During infection the influenza A virus NS1 protein participates in multiple protein-RNA and protein-protein interactions to perform a plethora of functions. The N-terminal 73 amino-acid residues of NS1 form a symmetrical homodimeric RNA-binding domain (RBD), which is connected to the central effector domain (ED; residues 86-204) via an inter-domain linker. Present models of the tertiary and quaternary structures of NS1 indicate that the protein possesses two globular domains, each capable of forming independent homodimeric interactions. Our bioinformatic analyses indicate that the N-terminal RBD forms a very stable homodimer, while the predominant and ubiquitous helix-helix contacts between C-terminal EDs bear many similarities with weak transient interfaces.

Previous studies using recombinant Alb/76 and Ud/72 EDs have shown that a single W187A amino-acid substitution is sufficient to prevent dimerization. However, as the strand-strand dimer has never been observed in structures from these strains, it may be that the PR8 ED behaves differently. We therefore introduced the W187A mutation into the PR8 NS1 ED bacterial expression construct. We crystallized the purified PR8 ED-W187A protein and solved the structure by molecular replacement. Two crystal forms were obtained for this protein, both occurring under the same crystallization condition but separated in time. Furthermore, the rationally-designed ‘helix-open’ NS1 protein (W187A) was poor at binding synthetic dsRNA, perhaps indicating that ED helix-helix dimeric interactions allosterically increase affinity of the RBD for dsRNA, or that ED homotypic interactions facilitate oligomerization of NS1 and thus cooperative binding to dsRNA.

>[2x]MTMASVPASRYLTDMTLEEMSRDWSMLIPKQKVAGPLCIRMDQAIMDKNIILKANFSVIFDRLETLILLRAFTEEGAIVGEISPLPSLPGHTAEDVKNAVGVLIGGLEANDNTVRVSETLQRFAWRSSNENGRPPLTPKQKREMAGTIRSEV>MRGSHHHHHHGSENLYFQGGSVLFGSLRGHVVGLRYYTGVVNNNE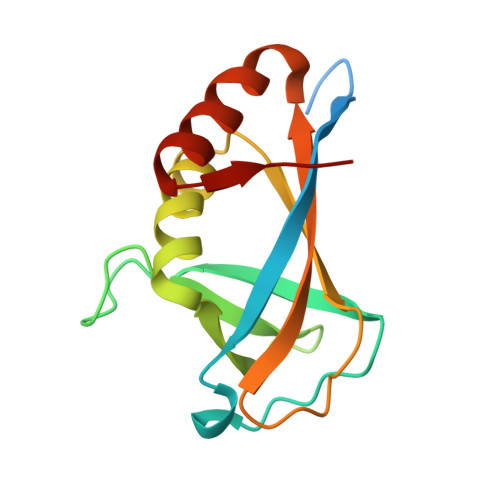MVALQRDPNNPYDKNAIKVNNVNGNQVGHLKKELAGALAYIMDNKLAQIEGVVPFGANNAFTMPLHMTFWGKEENRKAVSDQLKKHGFKLGPA[9x]6-bromo-7-hydroxy-2,2-dimethyl-2H,4H-1,3-benzodioxin-4-one | C10 H9 Br O4 | 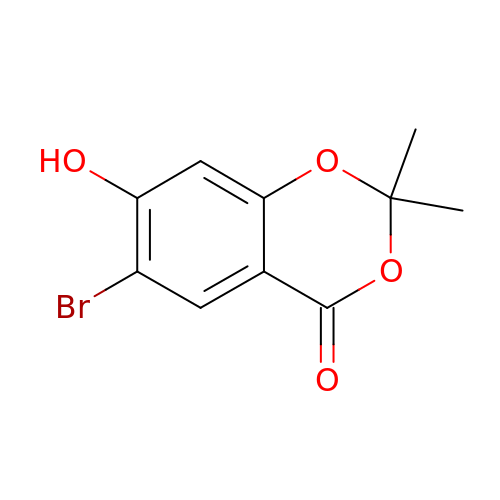FOZVJTHORLMHQD-UHFFFAOYSA-N DECYL(DIMETHYL)PHOSPHINE 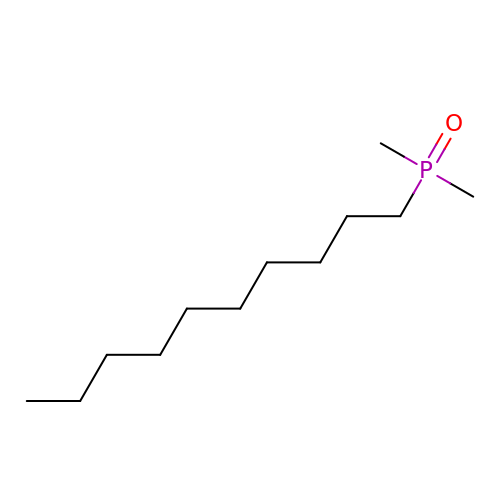OXIDE | C12 H27 O P | GSVLCKASFMVUSW-UHFFFAOYSA-N> GPHMKHPLMNVWTLWYLENDRSKSW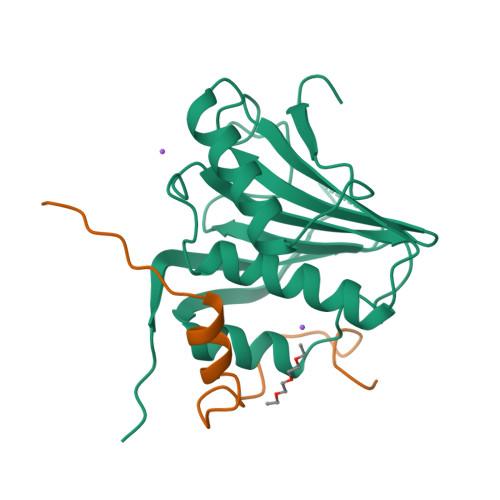EDMQNEITSFDTVEDFWSLYNHIKPPSEIKLGSDYSLFKKNIRPMWEDAANKQGGRWVITLNKSSKTDLDNLWLDVLLCLIGEAFDHSDQICGAVINIRGKSNKISIWTADGNNEEAALEIGHKLRDALRLGRNNSLQYQLHKDTMVKQGSNVKSIYTL;> GPHMTKLIYERAFMKNLRGSPLSQTPPSNVPSCLLRGT>APVKYGELIVLGYNGSLPNGDRGRRKSRFALFKRPKANGVKPSTVHIACTPQAAKAISNKDQHSISYTLSRAQTVVVEYTHDSNTDMFQIGRSTESPIDFVVTDTVPGSQSNSDTQSVQSTISRFACRIICE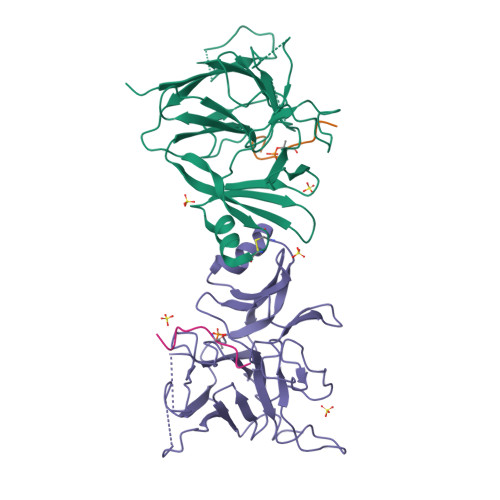RNPPFTARIYAAGFDSSKNIFLGEKAAKWKTSDGQMDGLTTNGVLVMHPRNGFTEDSKPGIWREISVCGNVFSLRETRSAQQRGKMVEIETNQLQDGSLIDLCGATLLWRTAEGLSHTP[2x];>[2x]AYEDSETQPFD>MAGIKIIKENVDRETFEALAEICPFDAFSYENDKLEVTAACKMCKMCLKKGPEGVLILEEDEKVAIDKSLYRGITVYVDHIEGQIHPVTFELIGKARELAAVIGHPVYALLMGTNITEKADELLKYGVDKVFVYDKPELKHFVIEPYANVLEDFIEKVKPSSILVGATNVGRSLAPRVAARYRTGLTADCTILEMKENTDLVQIRPAFGGNIMAQIVTENTRPQFCTVRYKVFTAPERVNEPWGDVEMMDIEKAKLVSAIEVMEVIKKEKGIDLSEAETIVAVGRGVKCEKDLDMIHEFAEKIGATVACTRPGIEAGWFDARLQIGLSGRTVKPKLIIALGISGAVQFAAGMQNSEYIIAINSDPKAPIFNIAHCGMVGDLYEILPELLTMIEGPENNKDTETISIPEAIETPERMVV[2x];>[2x]MSKILVCIKQVPGTSNVEVDPETGVLIRDGVESKLNPYDLFGLETAFRLKEQLGGTITTLSMGPMQSKEVLMESFYMGADEGCLLSDRKFGGADVVATSYTLAQGTKRLGDFDLIICGKQTTDGDTAQVGPEMAEFLGIPHVTNVIKILAADEKGLTLQMNMEESLEIQRVPYPCLITVDKDIYTPRLPSYKRKLDISKNPEIKILTLKDMYDTNEKKYGLSGSPTQVERIFPPESNVEKTSFEGDGKVLAKALLGILTEKKYLG;>[2x]MNYKKVEASDIAAIKELIPAERVFVGTEIGEDFSHDELGSIHSYPEVLIKVTSTEEVSKIMKYAYEHNIPVVVRGSGTGLVGACVPLFGGIMLETTLMNNILELDTENLTVTVEPGVLLMELSKFVEENDLFYPPDPGEKSATIAGNISTNAGGMRAVKYGVTRDYVRGLTVVLANGEIIELGGKIVKNSSGYSLKDLVIGSEGTLCVITKAILKLLPLPKMTLSLLIPFENISDAAGIVPKIIKSKAIPTAIEFMERQTILFAEDFLGKKFPDSSSNAYILLTFDGNTKEQVEAEYETVANLCLAEGAKDVYIVDTVERKDSVWSARGAFLEAIKASTTEMDECDVVVPRNRIAEFIEFTHDLAKEMDVRIPSFGHAGDGNLHIYVCRDELCQADWEAKLAEAMDRMYAKALTFEGLVSGEHGIGYAKRKYLLNDFGTEHLALMAGIKQTFDPKNLLNPKKVCQMA

The electron-confurcating lactate dehydrogenase/electron-transferring flavoprotein (Ldh-EtfAB) complex, the research subject of this report, catalyzes the endergonic oxidation of lactate to the central cellular metabolite pyruvate with NAD+ as electron acceptor driven by simultaneous co-oxidation of Fdred (Weghoff et al., 2015). This FBEC reaction occurs in anaerobic sulfate-reducing and acetogenic bacteria. The confurcating Ldh-EtfAB complex belongs to the bEtf family, the largest and most diverse group of FBEB/FBEC enzymes. bEtf family members are built up of a variable dehydrogenase/oxidoreductase core and several peripherally attached EtfAB modules (Demmer et al., 2018; Demmer et al., 2017; Feng et al., 2021). The EtfAB heterodimer is built up of an EtfAB base composed of the N-terminal segments of EtfA and EtfB (termed domains I and III, respectively) and a module termed domain II or EtfAB shuttle domain (due to its shuttling role between two sites far away from each other) formed by the tightly associated C-terminal segment of EtfA and the C-terminal arm of EtfB.

The electron cryo-microscopically characterized (Ldh-EtfAB)2 complex of Acetobacterium woodii at 2.43 Å resolution consists of a mobile EtfAB shuttle domain located between the rigid central Ldh and the peripheral EtfAB base units. The FADs of Ldh and the EtfAB shuttle domain contact each other thereby forming the D (dehydrogenation-connected) state. The cryo-EM structure of the fragile Ldh-EtfAB complex from A. woodii was determined from a sample cross-linked with bis(sulfosuccinimidyl)suberate (BS3), because multiple attempts without cross-linking failed. From 9,788 micrographs collected and 674,283 particles extracted a twofold-averaged density map at a mean resolution of 2.43 Å was calculated using Relion. The local resolution ranges from 2.3 Å for the Ldh core to 3.1 Å for a peripheral EtfA region. The EM density was only disordered for the N-terminal Fd domain (2-65) of EtfA, for which model building was impossible. In particular, the cryo-EM density at the flavin binding sites is highly reliable. The 255 kDa heterohexameric complex has an overall size of 150 Å x 100 Å x 60 Å. Lactate oxidation in Ldh is assisted by the catalytic base His423 and a metal center. The intermediary Glu37 and Glu139 may harmonize the redox potentials between the FADs and the pyruvate/lactate pair crucial for FBEC.>GPLGSKAPTVFSQNEASLLNQLKNIANREDYVVTWWDYGYPVRYYSDVKTLVDGGKHLGKDNFFPSFALSKDEQAAANMARLSVEYTEKSFYAPQNDILKSDILQAMMKDYNQSNVDLFLASLSKPDFKIDTPKTRDIYLYMPARMSLIFSTVASFSFINLDTGVLDKPFTFSTAYPLDVKNGEIYLSNGVVLSDDFRSFKIGDNVVSVNSIVEINSIKQGEYKITPIDDKAQFYIFYLKDSAIPYAQFILMDKTMFNSAYVQMFFLGNYDK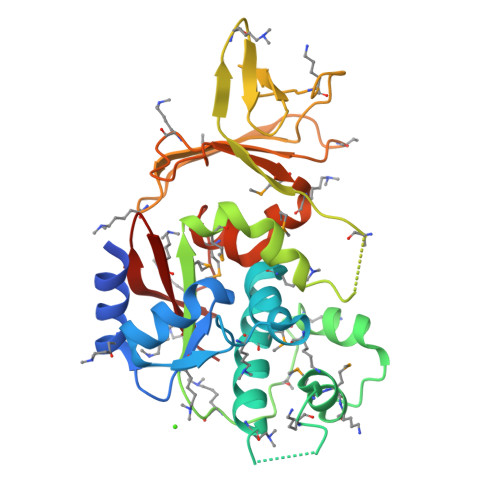NLFDLVINSRDAKVFKLKI[2x]> GSDKERFARSDDEQSSADKERLARENHSEIERRRRNKMTAYITELSDMVPTCSALARKPDKLTILRMAVSHMKSLRGTGNTSTDGSYKPSFLTDQELKHLILEAADGFLFIVSCETGRVVYVSDSVTPVLNQPQSEWFGSTLYDQVHPDDVDKLREQLSTSENALTGRILDLKTGTVKK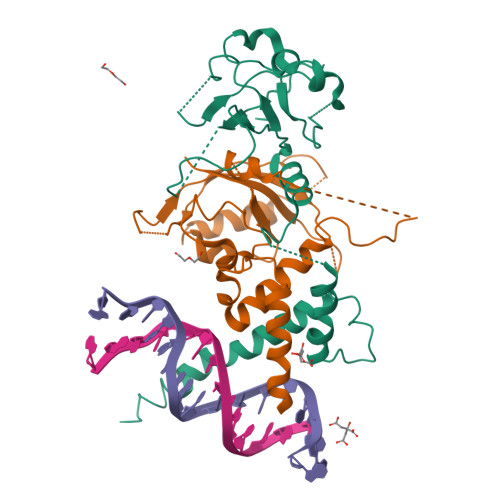EGQQSSMRMCMGSRRSFICRMRCGSSSVDPVSVNRLSFVRNRCRNGLGSVKDGEPHFVVVHCTGYIKAWPPAGVSLPDDDPEAGQGSKFCLVAIGRLQVT;> GSGIKSNPSKRHRDRLNTELDRLASLLPFPQDVINKLDKLSVLRLSVSYLRAKSFFDVALKSTPADRNGGQDQCRAQIRDWQDLQEGEFLLQALNGFVLVVTADALVFYASSTIQDYLGFQQSDVIHQSVYELIHTEDRAEFQRQLHWALNPDSAQGVDEAHGPPQAAVYYTPDQLPPENASFMERCFRCRLRCLLDNSSGFLAMNFQGRLKYLHGQNKKGKDGALLPPQLALFAIATPLQ>[2x]RGSMTIQDIQSLAEAHGLLLTDKM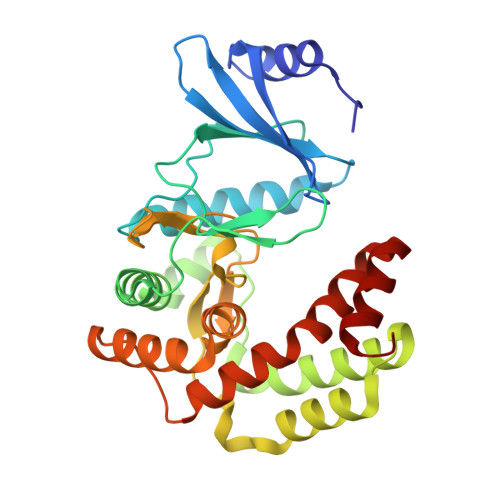NFNEMGIDFKVVFALDTKGQQWLLRIPRRDGMREQIKKEKRILELVKKHLSVEVPDWRISSTELVAYPILKDNPVLNLDAETYEIIWNMDKDSPKYITSLAKTLFEIHSIPEKEVRENDLKIMKPSDLRPEIANNLQLVKSEIGISEQLETRYRKWLDNDVLWADFTQFIHGDLYAGHVLASKDGAVSGVIDWSTAHIDDPAIDFAGHVTLFGEESLKTLIIEYEKLGGKVWNKLYEQTLERAAASPLMYGLFALETQNESLIVGAKAQLGVI6-(naphthalen-2-yl)-9-(5-O-phosphono-beta-D-ribofuranosyl)-9H-purine 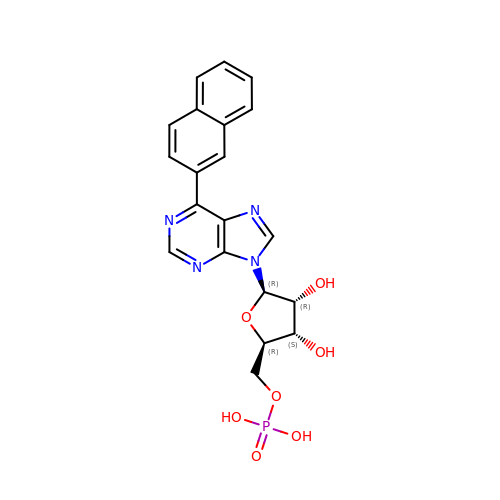| C20 H19 N4 O7 P | LQGRESLLVHYRLI-VXXKDZQQSA-N> GSHMLNTTYPESLSYPFGPDEGLALSESYTRARDTDGLIRVKLPYGEPAWLATRYEDARLVLGDARFSRALSEEHDPPRARKFNAQAKSMFNMDAPDHTRLRRLISKAFTIRRVEELRPKVHDLAHRLIDDMLAKGEPADLVADYA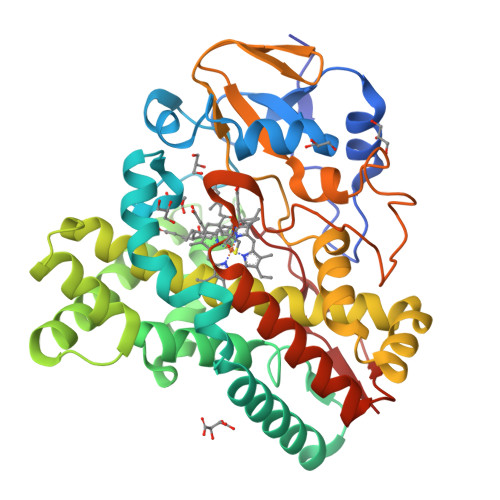LPIPTTVICELLGVPFEDREKFGRWTDAILSTSTLNPEEGRVKRMELVGYIGGIIAARRAQPADDLISGMIEARDVQDKLTEQELLDHCIGLLIAGHETTASQIPSFVYALLDQPQHWKRLLDDPELIPSAVEELFRFVPLGSGSAAPRYAREDIEVGGTLVRAGEPVLVALGAANRDGLRFEDPEEIKLDRPSNHHIGFGHGIHHCLGAPLARLELQEALRALLERLPTLKVAGDIAWKSEMMVRGPRSMPVGW>[2x]ATCDDGRTTANAACCILFPILDDIQENLFDGAQC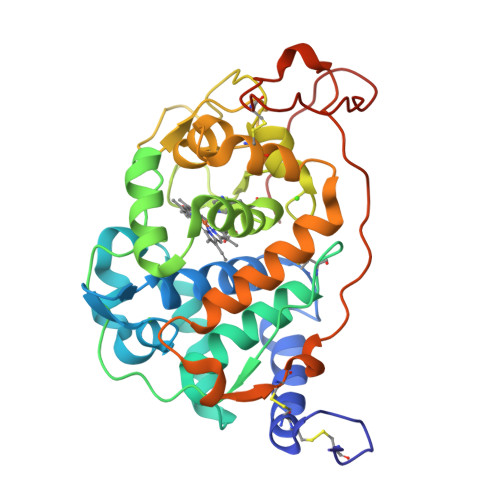GEKVRESLRLTFHDAIGFSPTLGGGGADGSIIAFDTIETNFPANAGIDEIVSAQKPFVAKHNISAGDFIQFAGAVGVSNCPGGVRIPFFLGRPDAVAASPDHLVPEPFDSVDSILARMGDAGFSPAEVVWLLASHSIAAADKVDPSIPGMPFDSTPGVFDSQFFIETLLKGRLFPGTAANKGEAQSPLQGEIRLQSDHLLARDPQTACEWQSMVNNQPKIQNRFAATMSKMALLGQDKTKLIDCSDVIPTPPALVGAAHLPAGFSLSDVEQACAATPFPALTADPGPVTSVPPVPRS> GSHMKNSVSVDLPGSMKVLVSKSSNADGKYDLIATVDALELSGTSDKNNGSGVLEGVKADASKVKLTISDDLGQTTLEVFKSDGSTLVSKKVTSGGSSTEEKGGEKIITRADGTRLEYTGIKSDGSGKAKEVLKGYVLEGTLTAEKTTLVVKEGTVTLSKNISKSGEVSVELNDTDSSAATKKTAAWNSGTSTLTITV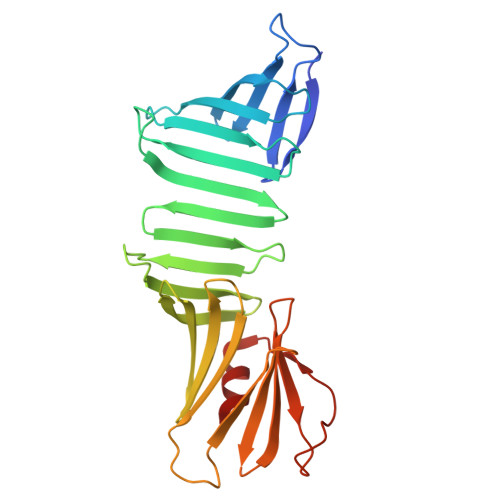NSKKTKDLVFTSSNTITVQQYDSNGTSLEGSAVEITKLDEIKNALK> GQGVVLPQPMPGIGQQMSPPKQQELDQLRKTAQLGTANAAKLLGSSTLLNKLAFASPEEFEIELSKMTSELEQTQKKLKLADLERIRAENLKKIDENQTKMKEASEAADKAKKS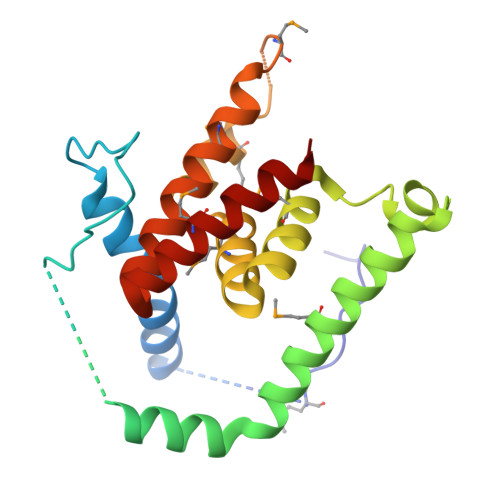GLASKIFGWISAIASMVIGAILIATGVGAAVGAMMIVGGAVGVANMAIQQAAADGRISPETMKVLGPIMIAAEILVAIVSIAVTFGASAASTAMKAVKFATQAAD>[2x]GAMASSNTAATNADSAWLEAQEEEEVGFPVRPQVPLRPMTYKAA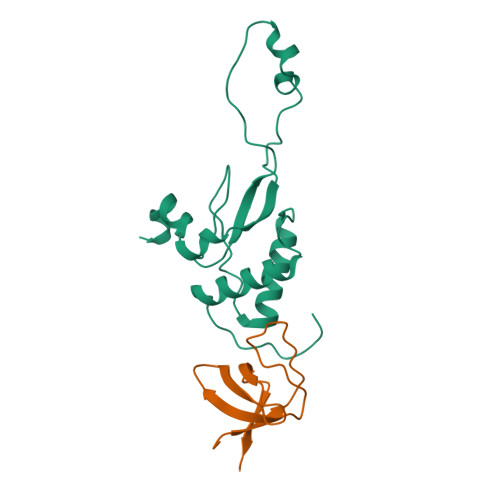LDISHFLKEKGGLEGLIWSQRRQEILDLWIYHTQGYFPDWQNYTPGPGIRYPLTFGWCFKLVPVEPEKVEEANEGENNSLLHPMSLHGMEDAEKEVLVWRFDSKLAFHHMARELHPEYYKDA;>[2x]MEDIIVVALYDYYSPFSWDLSFQKGDQMVVLEESGEWWKARSLATRKEGYIPSNYVARVDS> VHRKPSLLAHPGRLVKSEETVILQCWSDVRFEHFLLHREGKFKDTLHLIGEHHDGVSKANFSIGPMMQDLAGTYRCYGSVTHSPYQLSAPSDPLDIVITGLYEKPSLSAQPGPTVLAGESVTLSCSSRSSYDMYHLSREGEAHECRFSAGPKVNGTFQADFPLGPATHGGT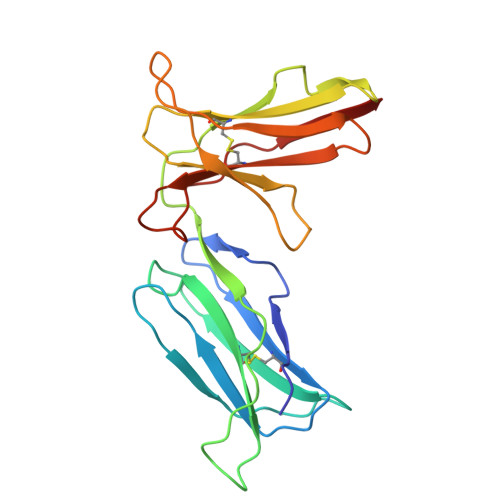YRCFGSFRDSPYEWSNSSDPLLVSVI>HMSIITDVYAREVLDSRGNPTLEVEVYTESGAFGRGMVPSGASTGEHEAVELRDGDKSRYLGLGTQKAVDNVNNIIAEAIIGYDVRDQQAIDRAMIALDGTPNKGKLGANAILGVSIAVARAAADYLEVPLYTYLGGFNTKVLPTPMMNIINGGSHSDAPIAFQEFMIMPVGAPTFKEGLRWGAEVFHALKKILKERGLVTAVGDEGGFAPKFEGTEDGVETILKAIEAAGYEAGENGIMIGFDCASSEFYDKERKVYDYTKFEGEGAAVRTSAEQVDYLEELVNKYPIITIEDGMDENDWDGWKVLTERLGKRVQLVGDDFFVTNTEYLARGIKENAANSILIKVNQIGTLTETFEAIEMAKEAGYTAVVSHRSGETEDSTIADIAVATNAGQIKTGSLSRTDRIAKYNQLLRI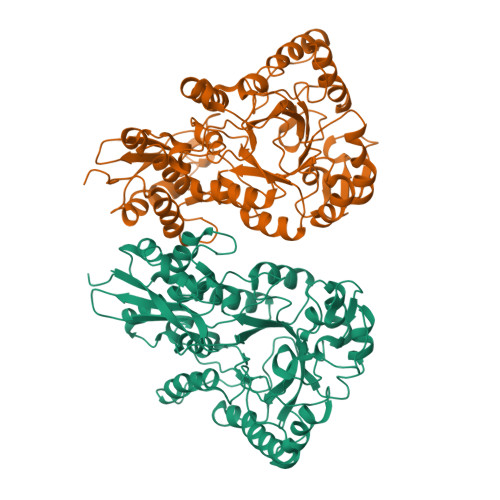EDQLGEVAQYKGIKSFYNLKK[2x]> MRSSILFLLKLMKIMDVQQQQEAMSSEDRFQELVDSLKPRTAHQYKTYYTKYIQWCQLNQIIPTPEDNSVNSVPYKDLPISAELIHWFLLDTLITDDKPGEKREETEDLDEEEENSFKIATLKKIIGSLNFLSKLCKVHENPNANIDTKYLESVTKLHTHWIDSQKAITTNETNNTNTQVLCPPLLKVSLNLWNPETNHLSEKFFKTCSEKLRFLVDFQLR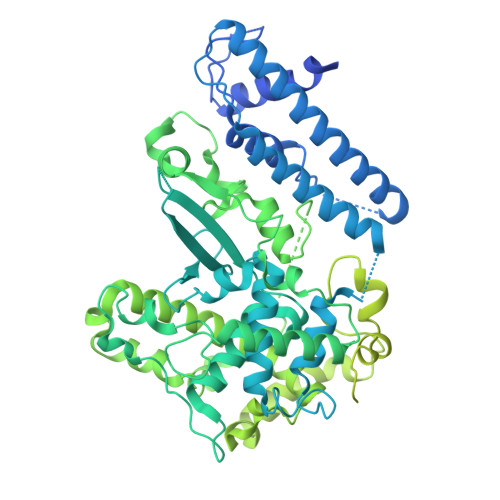SYLNLSFEERSKIRFGSLKLGKRDRDAIIYHKVTHSAEKKDTPGHHQLLALLPQDCPFICPQTTLAAYLYLRFYGIPSVSKGDGFPNLNADENGSLLQDIPILRGKSLTTYPREETFSNYYTTVFRYCHLPYKRREYFNKCNLVYPTWDEDTFRTFFNEENHGNWLEQPEAFAFPDKIPFDFKKIMNFKSPYTSYSTNAKKDPFPPPKDLLVQIFPEIDEYKRHDYEGLSQNSRDFLDLMEVLRERFLSNLPWIYKFFPNHDIFQDPIFGNSDFQSYFNDKTIHSKGSPILSFDILPGFNKIYKNKTNFYSLLIERPSQLTFASSHNPDTHPTQKQESEGPLQMSQLDTTQLNELLKQQSFEYVQFQTLSNFQILLSVFNKIFEKLEMKKSSRGYILHQLNLFKITLDERIKKSKIDDADKFIRDNQPIKKEENIVNEDGPNTSRRTKRPKQIRLLSIADSSDESSTEDSNVFKKDGESIEDGAYGENEDENDSEMQEQLKSMINELINSKISTFLRDQMDQFELKINALLDKILEEKVTRIIEQKLGSHTGKFSTLKRPQLYMTEEHNVGFDMEVPKKLRTSGKYAETVKDNDDHQAMSTTASPSPEQDQEAKSYTDEQEFMLDKSIDSIEGIILEWFTPNAKYANQCVHSMNKSGNKSWRANCEALYKERKSIVEFYIYLVNHESLDRYKAVDICEKLRDQNEGSFSRLAKFLRKWRHDHQNSFDGLLVYLSN> SMSDLH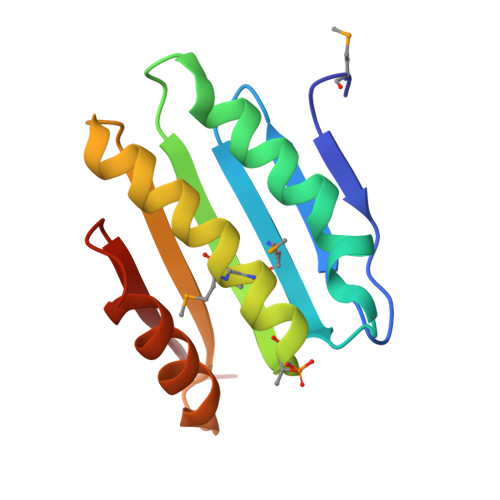IPGTQSTPAIQGDWQAGRLSMQGDSYPENSYELFGQVIDWVERFLADGQRPLELDLRLLYLNTSSIKAMMDILDLLEEAHQGGRPVSLRWHYDRRNERVAELAEEFREDCSFPFAIQAHDE Human noroviruses (huNoVs), members of the Norovirus genus of the Caliciviridae family, are the leading cause of acute gastroenteritis (AGE) and are associated with almost 20% of all AGE cases worldwide. The major capsid protein (VP1) is composed of a shell (S) domain and a protruding (P) domain, and the P domain is further divided into the P1 and P2 subdomains. The P2 subdomain is the main determinant of NoV diversity, antigenicity, and glycan binding patterns. In conclusion, GII.13/21 huNoVs have developed a novel GBS that interacts with glycans via the common β-Gal through a unique glycan binding mode.

A more important factor contributing to the low prevalence of the GII.13/21 huNoVs may be the GBS of the GII.13/21 huNoVs, which is easily interfered with. The function of the GII.13/21 GBSs appears to be easily blocked or inhibited by low-level glycerol molecules, suggesting that other small molecules with a glycine link structure also inhibit the GII.13/21 GBS. Indeed, we also detected a glycerol molecule in the GII.13 08N2045/2008 P dimer.

>TKSFTLPILTISEMTNSRFPIPIEQLYTAPNETNVVQCQNGRCTLDGELQGTTQLLSSAICSYRGRTLANNDSWDQNLLQLSYPNGASYDPTDEVPAPLGTQDFSGILYGVLTQDNVTEGTGEAKNAKGIYISTTSGKFTPKIGSIGLHSITGDVHHNQQSRFTPVGIAVNENTPFKQWVLPHYSGSLALNTNLAPAVAPTFPGEQLLFFRSRVPCVQGLHGQDAFIDCLLPQEWVNHFYQEAAPSQTDVALIRFVNPDTGRTLFEAKLHRSGFITVSHTGNYPLVIPPNGHFRFDSWVNQFYSLAPM[4x]>[2x]AFSVNYDSSFGGYSIHDYLGQWASTFGDVNHTNGNVTDANSGGFYGGSLSGSQYAISSTANQVTAFVAGGNLTYTLFNEPAHTLYGQLDSLSFGDGLSGGDTSPYSIQVPDVSF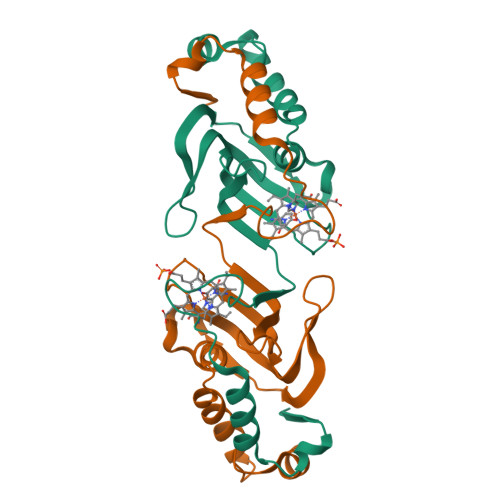GGLNLSSLQAQGHDGVVHQVVYGLMSGDTGALETALNGILDDYGLSVNSTFDQVAAATA>GPLGSMSSLSASAENVSSLGLGSGGGGTNSHDGNSQQGSGSDGGSSMCLELALEGERLCNAGDCRAGVAFFQAAIQAGTEDLRTLSAIYSQLGNAYFYLGDYNKAMQYHKHDLTLAKSMNDRLGEAKSSGNLGNTLKVMGRFDEAAICCERHLTLARQLGDRLSEGRALYNLGNVYHAKGKHLGQRNPGKFGDDVKEALTRAVEFYQENLKLMRDLGDRGAQGRACGNLGNTYYLLGDFQAAIEHHQERLRIAREFGDRAAERRANSNLGNSHIFLGQFEDAAEHYKRTLALAVELGEREVEAQSCYSLGNTYTLLHEFNTAIEYHNRHLAIAQELGDRIGEARACWSLGNAHSAIGGHERALKYAEQH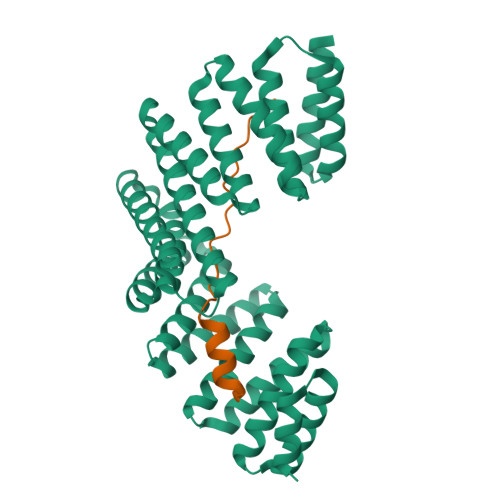LQLAXXXXXXXXXXXXXXXXXXXXXXXXXXXXXXXXXXXXXX[2x];>KRGKKHPEPVASWMSEQRWAGEPEVMCTLQHKSIAQEAYK[2x]> MKHHHHHHPMTTKQWGITPPISTAPATEQENALNTALINELKNQNLFESPAESEKRVKVLDELQQITTEFVKKVSLAKHMNEKMANEAGGKIFTYGSYRLGVYGPGSDIDTLVVVPKHVSRDNFFQDLEPMLREREEVTDLAAVPDAYVPIIKFKFLGISIDLIFARLSVPRVPRDLELSDNNLLKGVEERCVLSLNGTRVTDQILQLVPNRAVFKHALRAIKFWAQRRAIYANVVGFPGGVAWAMMVARICQL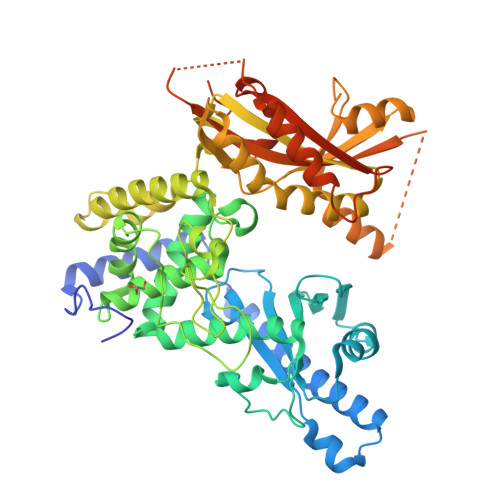YPNAVSSVIVAKFFRILHQWNWPQPILLKPIEDGPLQVRIWNPKLYPSDKAHRMPIITPAYPSMCATHNITLSTQTIILREMVRAGEIADQIMVKALPWSALFQKHDFFHRYKHYLTITAAAKTAEAQLKWAGLVESKLRHLVTRLELVDAIALAHPFNKGFDKVYNCSSEEEAQQVASGVTLEVAYESTDHEKLANDTVNEEKADNTESKADGSENGEKQIFPVYTTTCYIGLELEKKKGHPIKRLDISWPTQEFYELCKKWDKYDDTLMNVFIKNTKNTALPDEVFEPGEERPKATKKRSTADTAHSTEQLKRQKVSTA Mevaldyl-Coenzyme A | C27 H46 N7 O20 P3 S | 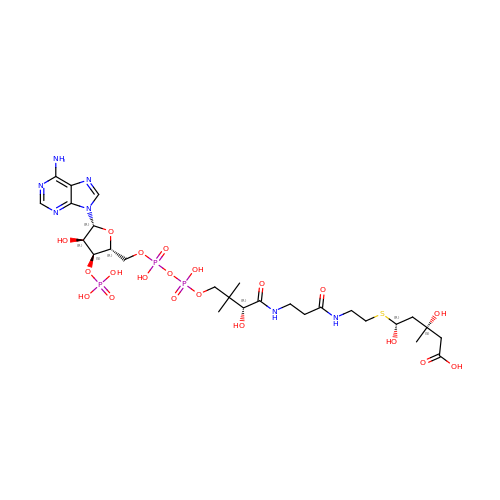RGCJQGNQJYHPPZ-NLYQEGKRSA-N>GNTVTIDFMSADGIVPGRTPVRYQGVEVGTVQDISLSDDLRKIEVKVSIKSDMKDALREETQFWLVTPKASLAGVSGLDALVGGNYIGMMPGKGKEQDHFVALDTQPKYRLDNGDLMIHLQAPDLGSLNSGSLVYFRKIPVGKVYDYAINPNKQGVVIDVLIERRFTDLVKKGSRFWNVSGVDANVSISGAKVKLESLAALVNGAIAFDSPEESKPAEAEDTFGLYEDLAHSQRGVIIKLELPSGAGLTADSTPLMYQGLEVGQLTKLDLNPGGKVTGEMTVDPSVVTLLRENTRIELRNPKLSLSDANLSALLTGKTFELVPGDGEPRKEFVVVPGEKALLHEPDVLTLTLTAPESYGIDAGQPLILHGVQVGQVIDRKLTSKGVTFTVAIEPQHRELVKGDSKFVVNSRVDVKVGLDGVEFLGASASEWINGGIRILPGDKGEMKASYPLYANLEKALENSLSDLPTTTVSLSAETLPDVQAGSVVLYRKFEVGEVITVRPRANAFDIDLHIKPEYRNLLTSNSVFWAEGGAKVQLNGSGLTVQASPLSRALKGAISFDNLSGASASQRKGDKRILYASETAARAVGGQITLHAFDAGKLAVGMPIRYLGIDIGQIQTLDLITARNEVQAKAVLYPEYVQTFARGGTRFSVVTPQISAAGVEHLDTILQPYINVEPGRGNP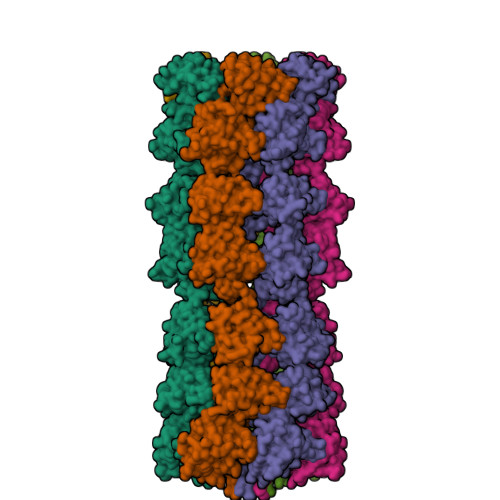RRDFELQEATITDSRYLDGLSIIVEAPEAGSLGIGTPVLFRGLEVGTVTGMTLGTLSDRVMIAMRISKRYQHLVRNNSVFWLASGYSLDFGLTGGVVKTGTFNQFIRGGIAFATPPGTPLAPKAQEGKHFLLQESEPKEWREWGTALPK[6x]>[3x]QMSSGEINKNYYQLPVVQSGTQSTASQGNRLLWVEQVTVPDYLAGNGVVYQTSDVKYVIANNNLWASPLDQQLRNTLVANLSTQLPGW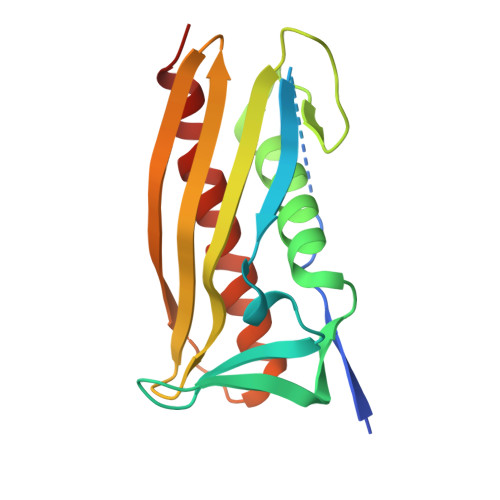VVASQPLGSAQDTLNVTVTEFNGRYDGKVIVSGEWLLNHQGQLIKRPFRLEGVQTQDGYDEMVKVLAGVWSQEAASIAQEIKRLP> QESSGNKIHFINVQEGGSDAIILESNGHFAMVDTGEDYDFPDGSDSRYPWREGIETSYKHVLTDRVFRRLKELSVQKLDFILVTHTHSDHIGNVDELLSTYPVDRVYLKKYSDSRITNSERLWDNLYGYDKVLQTATETGVSVIQNITQGDAHFQFGDMDIQLYNYENETDSSGELKKIWDDNSNSLISVVKVNGKKIYLGGDLDNVHGAEDKYGPLIGKVDLMKFNHHHDTNKSNTKDFIKNLSPSLIVQTSDSLPWKNGVDSEYVNWLKERGIERINAASKDYDATVFDIRKDGFVNISTSYKPIPSFQAGWHKSAYGNWWYQAPDSTGEYAVGWNEIEGEWYYFNQTGILLQNQWKKWNNHWFYLTDS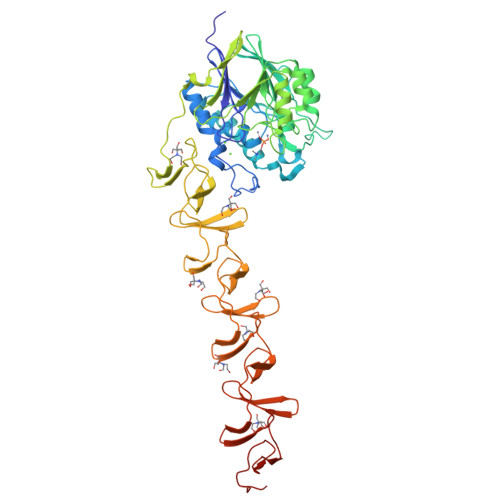GASAKNWKKIDGIWYYFNKENQMEIGWVQDKEQWYYLDVDGSMKTGWLQYMGQWYYFAPSGEMKMGWVKDKETWYYMDSTGVMKTGEIEVAGQHYYLEDSGAMKQGWHKKANDWYFYKTDGSRAVGWIKDKDKWYFLKENGQLLVNGKTPEGYTVDSSGAWLVDVSIEKSATIKTT> ENYLDLFSHKNMKLKERVLIPVKQYPKFNFVGKILGPQGNTIKRLQEETGAKISVLGKGSMRDKAKEEELRKGGD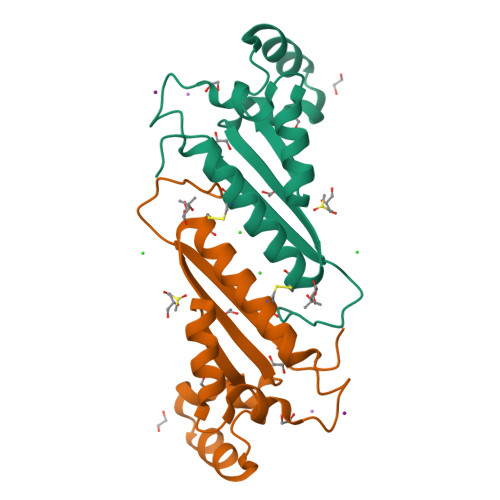PKYAHLNMDLHVFIEVFGPPCEAYALMAHAMCEVKKFLVPDMM(2R)-4-[4-(2-fluoro-4-methoxyphenyl)-2-oxopyridin-1(2H)-yl]-N-hydroxy-2-methyl-2-(methylsulfonyl)butanamide 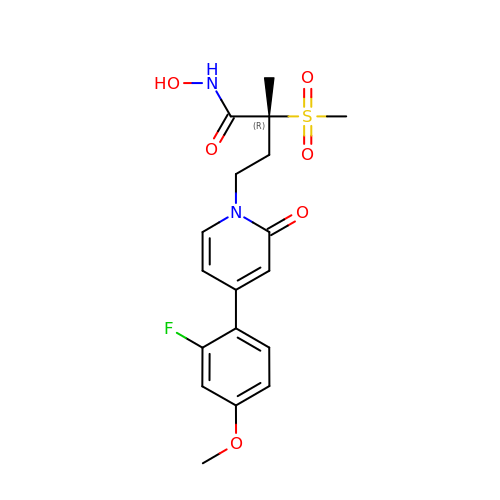| C18 H21 F N2 O6 S | DNVUWHWBCMGQLU-GOSISDBHSA-N>[4x]MKNNGGARVVVIGAGFV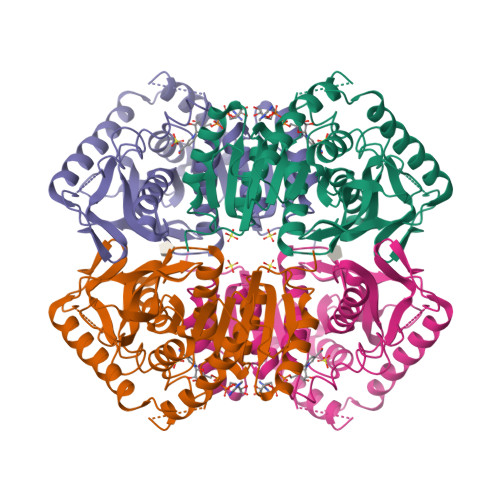GASYVFALMNQGIADEIVLIDANESKAIGDAMDFNHGKVFAPKPVDIWHGDYDDCRDADLVVICAGANQKPGETRLDLVDKNIAIFRSIVESVMASGFQGLFLVATNPVDILTYATWKFSGLPHERVIGSGTILDTARFRFLLGEYFSVAPQNVHAYIIGEHGDTELPVWSQAYIGVMPIRKLVESKGEEAQKDLERIFVNVRDAAYQIIEKKGATYYGIAMGLARVTRAILHNENAILTVSAYLDGLYGERDVYIGVPAVINRNGIREVIEIELNDDEKNRFHHSAATLKSVLARAFTR PANTOTHENYL-AMINOETHANOL-11-PIVALIC ACID | C16 H30 N2 O6 | 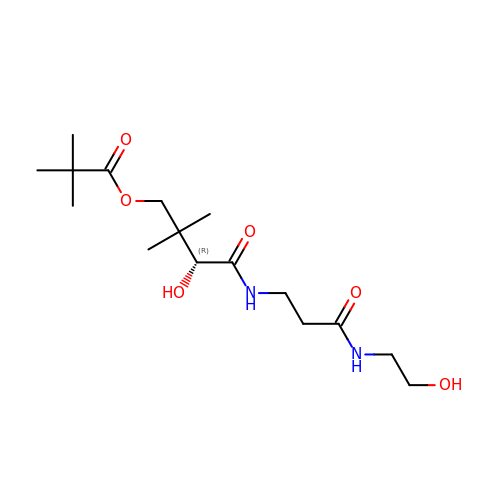BUEKNBNKVUKNIB-LBPRGKRZSA-N>[4x]AFDALREPDRESSAPPDDVQLVPGARIANGRYRLLIFHGGVPPLQFWQALDTALDRQVALTFVDPQGVLPDDVLQETLSRTLRLSRIDKPGVARVLDVVHTRAGGLVVAEWIRGGSLQEVADTSPSPVGAIRAMQSLAAAADAAHRAGVALSIDHPSRVRVSIDGDVV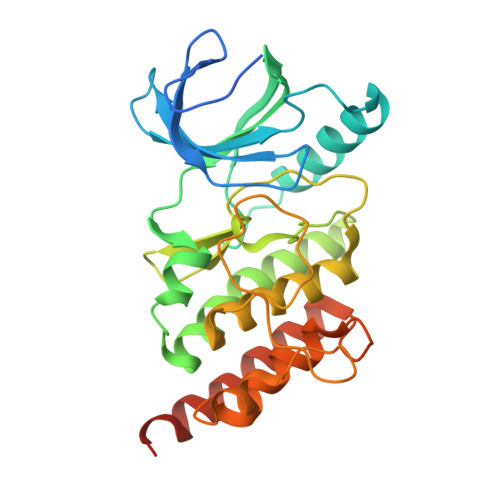LAYPATMPDANPQDDIRGIGASLYALLVNRWPLPEAGVRSGLAPAERDTAGQPIEPADIDRDIPFQISAVAARSVQGDGGIRSASTLLNLMQQATAVADRTEVLGPIDEAPVSAAPR>MKKYTCTVCGYIYNPEDGDPDNGVNPGTDFKDIPDDWVCP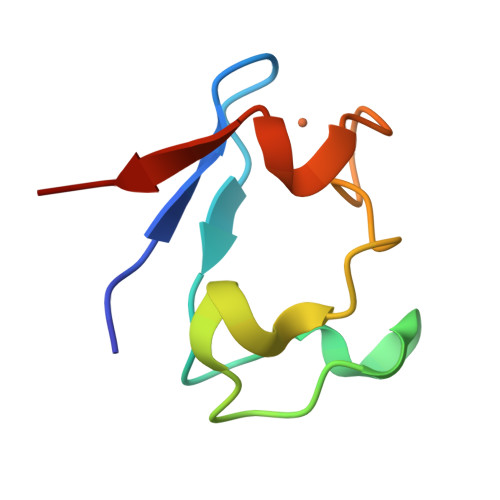LCGGGKDQFEEVEE[3x]>AYSNTYQEFTNIDQAKAWGNAQYKKYGLSKSEKEAIVSYTKSASEINGKLRQNKGVINGFPSNLIKQVELLDKSFNKMKTPENIMLFRGDDPAYLGTEFQNTLLNSNGTINKTAFEKAKAKFLNKDRLEYGYISTSLMNVS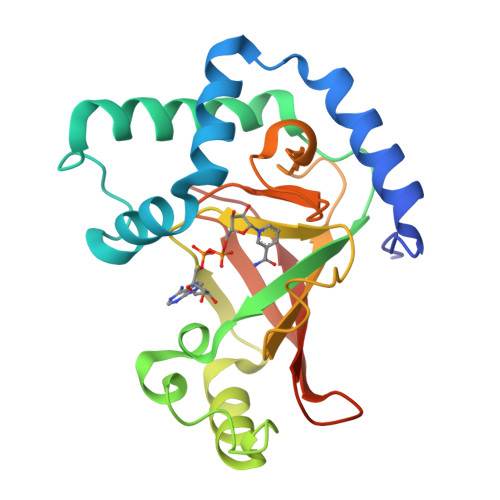QFAGRPIITKFKVAKGSKAGYIDPISAFAGALEMLLPRHSTYHIDDMRLSSDGKQIIITATMMGTAINPK[4x]> GPDSMSDIKQLLKEAKQELTNRDYEETIEISEKVLKLDPDNYFAHIFLGKALSSLPASNNVSSNRNLERATNHYVSAAKLVPDNLLAWKGLFLLFRTTEVVPDILSYDEYFDLCGQYADALLKQEQSQVELINDIKLLKKTHPDCQKAFYQHLKPGSLMAETIGRHLSTPQDALLNLIKILSNIETTEIGKTLSQNRLKLKASDPDYQIKLNSFSWEIIKNSEIDQLYNQLVNILADDQKRSEIENQWLEYRIKVLKSMPLDVKKDFFTKVKEMVEDMVLVNHQSLLAWQKYFEWTDYEDLDNMDAPLIIKYFKKFPKDPLAMILYSWLSSKLSKYDIKSLESANKPPEGHKKTEKETDIKDVDETNEDEVKDRVEDEVKDRVEDEVKDQDEEAKEDEEEDLDDIEIGLLEEEVVTVLTENIVKCKNNILAHRILCQYYLLTKEYEAALPYIKNGISLIAYNIKDLGVHLPLTKREFSLDLATVYTYVDAPKDHNAALKLYDNILSGDFSNIQAKMGKGIIFIERKNWKDAMTLLTQVHEQSPNNLEVLSELSWSKAHMGYMDEALAGLDTVIKGIKGMDLRSIDFRALNLWRQAKVYIMKHASINDAKQENVKCAFKLLIQSIKILDTFAPGFSTLGDIYCHYYKDHLRAFKCYFKAFDLDAGDYTAAKYITETYASKPNWQAASSIASRLIKGEKAKAELRSNNWPFRVVGIAHLEKQEESDSIEWFQSALRVDPNDVESWVGLGQAYHACGRIEASIKVFDKAIQLRPSHTFAQYFKAISLCDVGEYLESLDILEKVCQEAATEESFQIGLVEVLMRCSLDLYSQGFLLKSVSIAKDTIERIKIIISELKCENQQVWIYLSQVLRLFIWIESKVDTLPVESLVSIFENSQFSGSEEIDSVDNIKIDTLLDSTTDDNVSIACKFLILASKYSVSDQKFTDIAGTVRASYWYNIGISELTAFITLKEPQYRDAAIFAFKKSIQLQSNTSETWIGLGIATM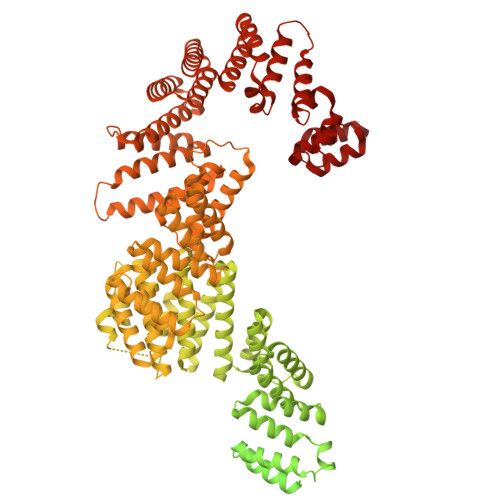DINFRVSQHCFIKATALEPKATNTWFNLAMLGLKKKDTEFAQQVLNKLQSLAPQDSSPWLGMALILEEQGDIIGSSKLFAHSFILSNGRSKAAQFMYAKNVLENHINNGDDERDIETVEKLTTASIALEQFFKKSPDSQFALQCALLTLERLHHYENANELANRLIGILEKKFEKTQDERELFNFAIIKGQFARIHLGLGNFELSIENADLSQGIISESSDEKSMKTKISNHICLGLSYFFLNDFDQTLNQFQELLSISKDSKHLVVLIAKVLYDVGESDTKEIALQELTEYIATSGADLLVTLTIAAMSILDDKREDLSIILEELKALPLSKQIIDKHKDAPYLIEEITKRLYRNDTGKQVWQRSAYFFPNNLKVWERLDKNIQRRIASNGQNKVTAEEMSKLYCESKNLRSIQRGMFLCPWNVTAVKALNECF>SSVILTNYMDTQYYGEIGIGTPPQTFKVVFDTGSSNVWVPSSKCSRLYTACVYHKLFDASDSSSYKHNGTELTLRYSTGTVSGFLSQDIITVGGITVTQMFGEVTEMPALPFMLAEFDGVVGMGFIEQAIGRVTPIFDNIISQGVLKEDVFSFYYNRDSENSQSLGGQIVLGGSDPQHYEGNFHYINLIKTGVWQIQMKGVSVGSSTLLCEDGCLALVDTGASYISGSTSSIEKLMEALGAKKRLFDYVVKCNEGPTLPDISFHLGGKEYTLTSADYVFQESYSSKKLCTLAIHAMDIPPPTGPTWALGATFIRKFYT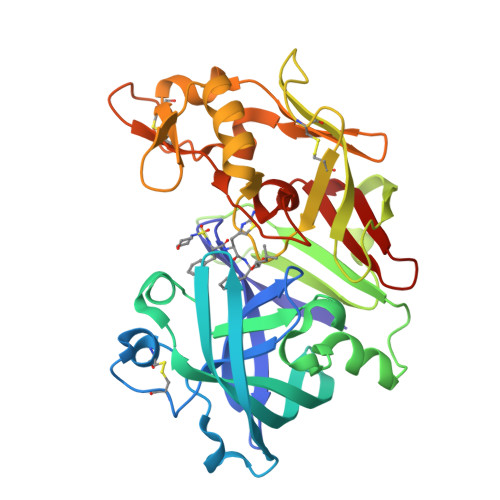EFDRRNNRIGFALAR[2x]>MVEPGRYRVINVKGGTALDLDINNNSTVHGWAFHGGDNQLWDFEHIGDNIWTICNANTGGYLAIVNGIAGDGVKAVSWADPFEWAVWPDENDGSVWRIGVPDTAFHLDLSDHGNSADGTAVQVWNASDGRNQCWVVEEA[2x]

We introduce a new family of fungal protease inhibitors with β-trefoil fold from the mushroom Coprinopsis cinerea, named cocaprins, which inhibit both cysteine and aspartic proteases. Cocaprins are small proteins (15 kDa) with acidic isoelectric points that form dimers. Cocaprins inhibit plant C1 family cysteine proteases with Ki in the micromolar range, but do not inhibit the C13 family protease legumain, which distinguishes them from mycocypins. Cocaprins also inhibit the aspartic protease pepsin with Ki in the low micromolar range.

CCP1 crystallized in P21 space group with two molecules in the asymmetric unit. CCP1 has a β-trefoil fold, consisting of only β-strands. The fold resembles a tree with a six-stranded β-barrel as a stem and additional three pairs of β-strands and connecting loops as the tree crown. The three-dimensional structure of cocaprin 1 showed similarity to fungal β-trefoil lectins. Based on the crystal structure, we designed mutations in the surface exposed loops, which were of sufficient length to be able to inhibit aspartic and cysteine proteases. Equilibrium constants were determined for the inhibition of papain and pepsin, which indicated that the β2-β3 loop containing the N22R mutation was involved in papain inhibition because this mutant had an approximately ten-fold higher Ki value. Since the same mutant had a Ki value for pepsin inhibition comparable to that of the wild type CCP1, this suggests that the inhibitory reactive sites for aspartic and cysteine proteases are located at different positions on the protein. Only the N22 mutation in CCP1 significantly reduced its ability to inhibit cysteine proteases, suggesting that the β2-β3 loop is critical for inhibition, which is different from that of clitocypin. The corresponding loop in CCP1 is much shorter and consists of only five residues (Val99-Ala103). It makes a rather tight turn between β strands β9 and β10 and does not protrude from the globular core of the protein, so it is unlikely to be involved in aspartic protease inhibition.>MLIAVPLDDTNFSENLKKAKEKGADIVELRVDQFSDTSLNYVKEKLEEVHSQGLKTILTIRSPEEGGREVKNREELFEELSPLSDYTDIELSSRGLLVKLYNITKEAGKKLIISYHNFELTPPNWIIREVLREGYRYGGIPKIAVKANSYEDVARLLCISRQVEGEKILISMGDYGKISRLAGYVFGSVITYCSLEKAFAPGQIPLEEM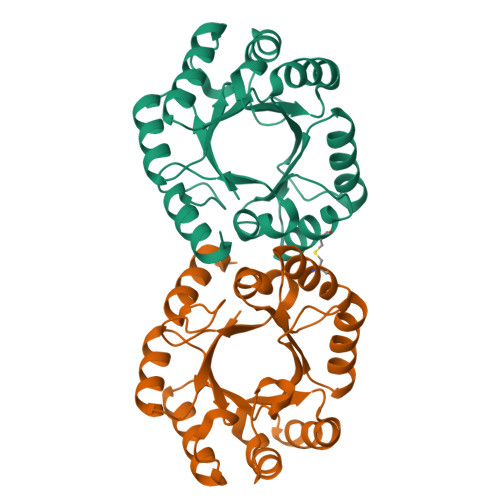VELRKKFYRL[3x]> GPLGSIYSPHETLAEKHSEKKLMDSFSPSLSQDKMDGEFAHANIDGISIRLCLNKGICSVFYLDGDKIQSTQLSSKEYNNLLSSLPPKQFNLGKVHTITAPVSGNFKTHKPAPEVIETAINCCTSIIPNDDYFHVKDTDFNSVWHDIYRDIRASDSNSTKIYFNNIEI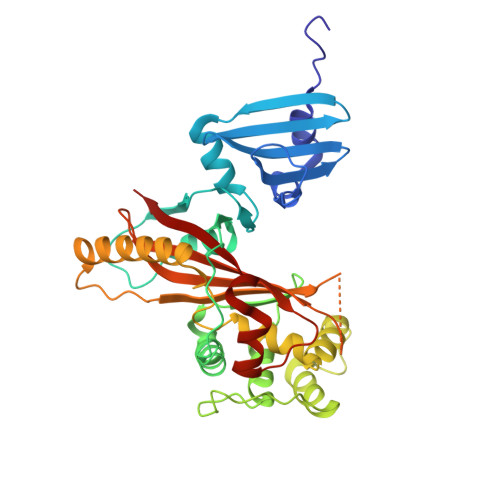PLKLIADLINELGINEFIDSKKELQMLSYNQVNKIINSNFPQQDLCFQTEKLLFTSLFQDPAFISALTSAFWQSLHITSSSVEHIYAQIMSENIENRLNFMPEQRVINNCGHIIKINAVVPKNDTAISASGGRAYEVSSSILPSHITCNGVGINKIETSYLVHAGTLPSSEGLRNAIPPESRQVSFAIISPDV3-FLUORO-2-(PHOSPHONOOXY)PROPANOIC ACID | C3 H6 F O6 P | 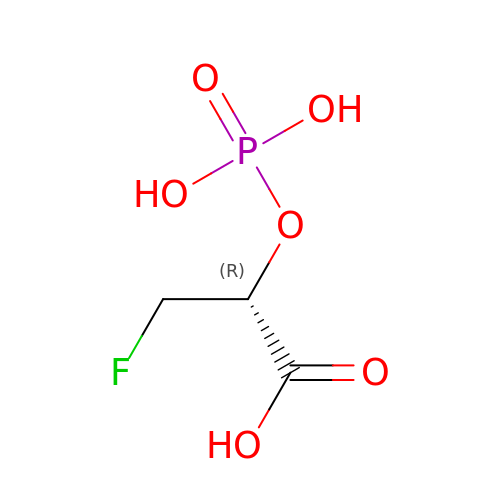BNOCDEBUFVJMQI-REOHCLBHSA-N3-[2-(2-hydroxyphenyl)ethyl]-5-methoxy-phenol 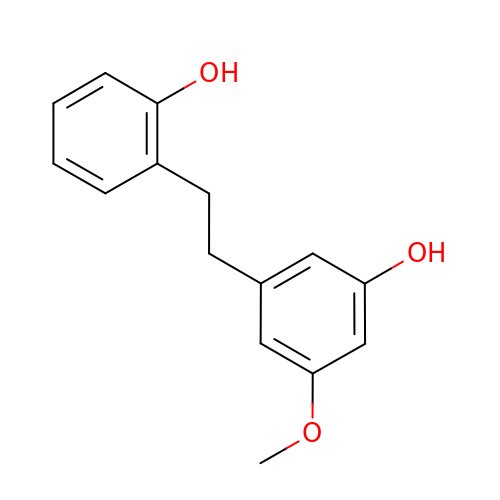| C15 H16 O3 | IUMFLNFLJUUODE-UHFFFAOYSA-N> IVDRAKMGDTLKRRFFYDQAFAIYGGVSGLYDFGPVGCALKNNIIQTWRQHFIQEEQILEIDCTMLTPEPVLKTSGHVDKFADFMVKDVKNGERFRADHLLKAHLQKLMSDKKCSVEKKSEMESVLAQLDNYGQQELADLFVNYNVKSPITGNDLSPPVSFNLMFKTFIGPGGNMPGYLRPETAQGIFLNFKRLLEFNQGKLPFAAAQIGNSFRNEISPRSGLIRVREFTMAEIEHFVDPSEKDHPKFQNVADLHLYLYSAKAQVSGQSARKMRLGDAVEQGVINNTVLGYFIGRIYLYLTKVGISPDKLRFRQHMENEMAHYACDCWDAESKTSYGWIEIVGCADRSCYDLSCHARATKVPL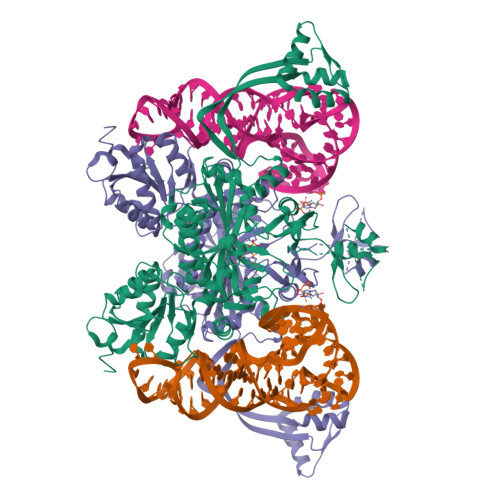VAEKPLKEPKTVNVVQFEPSKGAIGKAYKKDAKLVMEYLAICDECYITEMEMLLNEKGEFTIETEGKTFQLTKDMINVKRFQKTLYVEEVVPNVIEPSFGLGRIMYTVFEHTFHVREGDEQRTFFSFPAVVAPFKCSVLPLSQNQEFMPFVKELSEALTRHGVSHKVDDSSGSIGRRYARTDEIGVAFGVTIDFDTVNKTPHTATLRDRDSMRQIRAEISELPSIVQDLANGNITWADVEARYPLFEGQETGKKETIEELEHHHHHH> GSEFVKEHDWKKCDQSGFCRRNRAYADHALSAISWESPYKIAPETGSFKDGQYQAIILKTINDHGETVRLPLTVSFLESGTARVTIDEEKRQKGEIELRHDSKARKERYNEAEQWVIVGGMTLDKGAKVDYEDKTQMTVKYGPSSKFEATIKFAPFSIDFKRDGASHIKFNDQGLLNIEHWRPKIDPPPEPEKKEGEQQPDKKEEAPREDDSTWWEESFGGNTDSKPRGPESVGLDISFVGYEHVFGIPSHASPLSLKQTRGGEGNYNEPYRMYNADVFEYILDSPMTLYGSIPFMQAHRKDSSVGIFWLNAAETWVDITKGKDSKNPLALGVKSKITTRTHWFSESGLLDVFVFLGPTPKDIISKYAELTGTTAMPQEFSLGYHQCRWNYVSDEDVKDVDRKMDKFNMPYDVIWLDIEYTDEKKYFTWDKHSFKDPIGMGKQLEAHGRKLVTIIDPHIKNTNNYPVVDELKSKDLAVKTKDGSIFEGWCWPGSSHWIDAFNPAAREWWKGLFKYDKFKGTMENTFIWNDMNEPSVFNGPEVTMPKDNLHHGNWEHRDVHNLNGMTFQNATYHALLSRKPGEHRRPFVLTRAFFAGSQRLGAMWTGDNTADWGYLKASIPMVLSQGIAGFPFAGADVGGFFGNPDKDLLTRWYQTGIFYPFFRAHAHIDARRREPYLTGEPYNTIIAAALRLRYSLLPSWYTAFRHAHLDGTPIIKPMFYTHPSEEAGLPIDDQFFIGNTGLLAKPVTDKDRTSVDIWIPDSEVYYDYFTYDIISAAKSKTATLDAPLEKIPLLMRGGHVFARRDIPRRSSALMKWDPYTLVVVLGNDRKAEGDLYVDDGDSFDYEKGQYIHRRFIFDANTLTSADYEGRDDASIKEGEWLKKMRTVNVEKIIVVGAPAAWKGKKTVTVESEGKTWAAAIEYNPAEKSRAAFAVVKKVGVRVGAD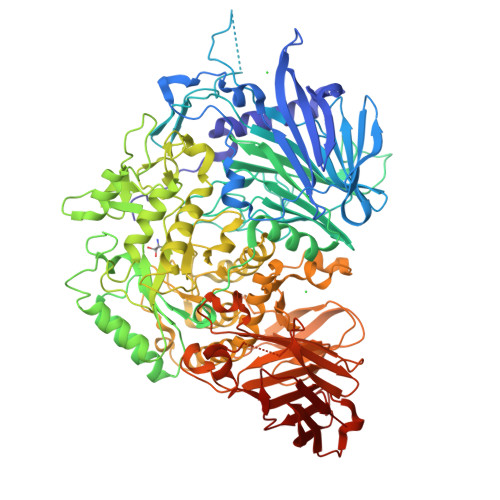FKIVFG> EDELYRQSLEIISRYLREQATGAKDTKPMGRSG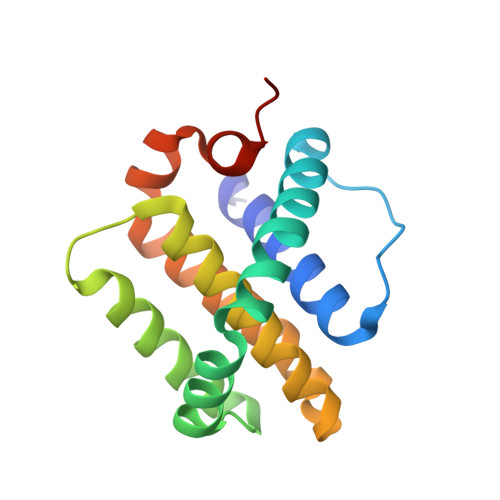ATSRKALETLRRVGDGVQRNHETAFQGMLRKLDIKNEDDVKSLSRVMIHVFSDGVTNWGRIVTLISFGAFVAKHLKTINQESCIEPLAESITDVLVRTKRDWLVKQRGWDGFVEFFHVEDLEGG> MMRKLKTLPPTLRDKNR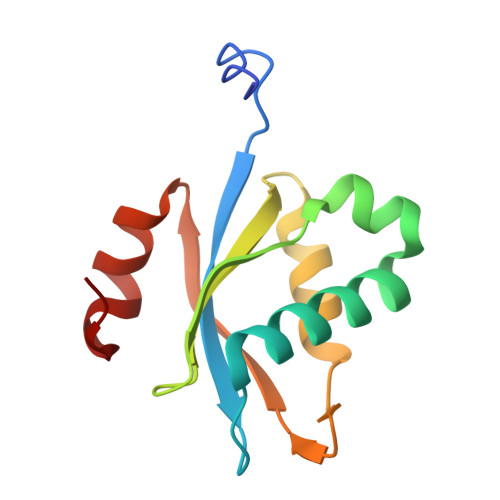YIAFEIISDGDFTKDEVKELIWKSSLEVLGETGTAIVKPWLIKFDPNTKTGIVRSDREYVEYLRFALMLVSEFNGKRLIIRTLGVSGTIKRLKRKFLAKYGWK> DLTVKEKEELIEEWQPEPLVPPVPKDHPALNYNIVSGPPSHKTVVNGKECINFASFNFLGLLDNPRVKAAALASLKKYGVGTCGPRGFYGTFDVHLDLEDRLAKFMKTEEAIIYSYGFATIASAIPAYSKRGDIVFVDRAACFAIQKGLQASRSDIKLFKHNDMADLERLLKEQEIEDQKNPRKARVTRRFIVVEGLYMNTGTICPLPELVKLKYKYKARIFLEESLSFGVLGEHGRGVTEHYGINIDDIDLISANMENALASIGGFCCGRSFVIDHQRLSGQGYCFSASLPPLLAAAAIEALNIMEENPGIFAVLKEKCGQIHKALQGISGLKVVGESLSPAFHLQLEESTGSREQDVRLLQEIVDQCMNRSIALTQARYLEKEEKCLPPPSIRVVVTVEQTEEELERAASTIKEVAQAVLL;> MRPEPGGCCCRRTVRANGCVANGEVRNGYVRSSAAAAAAAAAGQIHHVTQNGGLYKRPFNEAFEETPMLVAVLTYVGYGVLTLFGYLRDFLRYWRIEKCHHATEREEQKDFVSLYQDFENFYTRNLYMRIRDNWNRPICSVPGARVDIMERQSHDYNWSFKYTGNIIKGVINMGSYNYLGFARNTGSCQEAAAKVLEEYGAGVCSTRQEIGNLDKHEELEELVARFLGVEAAMAYGMGFATNSMNIPALVGKGCLILSDELNHASLVLGARLSGATIRIFKHNNMQSLEKLLKDAIVYGQPRTRRPWKKILILVEGIYSMEGSIVRLPEVIALKKKYKAYLYLDEAHSIGALGPTGRGVVEYFGLDPEDVDVMMGTFTKSFGASGGYIGGKKELIDYLRTHSHSAVYATSLSPPVVEQIITSMKCIMGQDGTSLGKECVQQLAENTRYFRRRLKEMGFIIYGNEDSPVVPLMLYMPAKIGAFGREMLKRNIGVVVVGFPATPIIESRARFCLSAAHTKEILDTALKEIDEVGDLLQLKYSRHRLVPLLDRPFDETTYEETED;> MADYKDDDDKSGPDEVDASGRMAGMALARAWKQMSWFYYQYLLVTALYMLEPWERTVFNSMLVSIVGMALYTGYVFMPQHIMAILHYFEIVQ;> MVGTAHSEVNPNTRVMNSRGIWLSYVLAIGLLHIVLLSIPFVSVPVVWTLTNLIHNMGMYIFLHTVKGTPFETPDQGKARLLTHWEQMDYGVQFTASRKFLTITPIVLYFLTSFYTKYDQIHFVLNTVSLMSVLIPKLPQLHGVRIFGINKY;> MATATEQWVLVEMVQALYEAPAYHLILEGILILWIIRLLFSKTYKLQERS

The ORM/ORMDL family proteins function as regulatory subunits of the serine palmitoyltransferase (SPT) complex, which is the initiating and rate-limiting enzyme in sphingolipid biosynthesis. In humans, the heterotrimeric SPT core enzymatic complex, composed of SPTLC1, SPTLC2 or SPTLC3, and SPTssa or SPTssb, catalyzes the first and rate-limiting step of de novo sphingolipid biosynthesis by condensation of serine and palmitoyl-CoA to generate 3-keto-dihydrosphingosine (3-KDS). As a critical mechanism for the homeostatic regulation of sphingolipid production, SPT activity is inhibited in response to elevated cellular sphingolipid levels in an ORM/ORMDL-dependent manner. In this work, we demonstrate that ceramide binds directly with and inhibits the human SPT-ORMDL complexes, a process that is important for establishing cellular sphingolipid homeostasis.

To investigate how ORMDL3 N-terminal mutations release SPT inhibition by ORMDL3 and disturb C6-ceramide-mediated SPT-ORMDL3 inhibition, we determined the structure of SPT-ORMDL3 variant bearing ORMDL3-ΔN2 mutation at an overall resolution of 3.1 Å for the monomeric complex. Although the overall structure of ORMDL3-ΔN2 mutant is closely identical to that of the WT complex, the N-terminal segment of ORMDL3-ΔN2 is disordered, rather than inserted into the substrate binding site as it is in the WT structure. This supports a vital role of Asn2 in stabilizing the ORMDL3 N-terminus. The fixed N-terminus of ORMDL3 in the WT SPT-ORMDL3 complex presumably prevents the binding of palmitoyl-CoA to the enzyme. This is supported by the increased Khalf for palmitoyl-CoA in the ORMDL3-containing complex, whereas the flexible N-terminus of ORMDL3-ΔN2 would permit substrate binding, thus liberating SPT from ORMDL3 inhibition. In addition to the dissimilarities at the ORMDL3 N-terminus, the ceramide-like density sandwiched between ORMDL3 and SPTLC2 in the WT complex was largely diminished in the ORMDL3-ΔN2 mutant, suggesting that this mutation weakens ceramide binding. In line with this, the ORMDL3-ΔN2 mutation causes some local conformational changes for the residues near the ceramide binding pocket, especially Asn13 of ORMDL3, which would be expected to affect ceramide binding. Accordingly, the ceramide-enrichment from the purified ORMDL3-ΔN2 mutant was approximately 25% lower than that of the WT complex. The Asn2 of ORMDL3 forms a hydrogen bond with the main chain of Leu330 in SPTLC1. Mutation of Asn2 of ORMDL3 to alanine achieved effects similar to that of the ORMDL3 N-terminal deletion mutants, supporting the importance of the polar interaction between ORMDL3 N-terminus and SPTLC1. The remaining 75% may largely represent ceramide, along with other membrane lipids, bound to the detergent micelles in the isolated complex, or, some other potential ceramide binding sites in the complex. These results suggest that there is an important interplay between the N-terminus of ORMDL3 and the ceramide binding site.> EANEGSKTLQRNRKMAMGRKKFNMDPKKGIQFLVENELLQNTPEEIARFLYKGEGLNKTAIGDYLGEREELNLAVLHAFVDLHEFTDLNLVQALRQFLWSFRLPGEAQKIDRM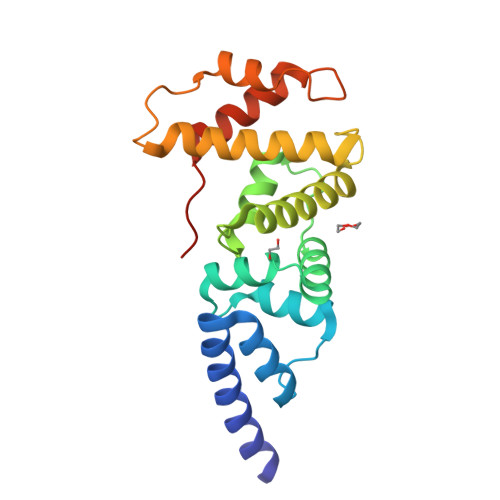MEAFAQRYCLCNPGVFQSTDTCYVLSFAVIMLNTSLHNPNVRDKPGLERFVAMNRGINEGGDLPEELLRNLYDSIRNEPFKIPEDDGND> APSRANTKVIVVGGGGTIGSSTALHLVRSGYTPSNVTVLDAYPIPSCQSAGNDLNKIMDADADPAADAARQMWNEDELFKKFFHNTGRLDCAHGEKDIADLKKRYQNLVDWGLDATVEWLDSEDEILKRMPQLTRDQIKGWKAIFSKDGGWLAAAKAIKAIGEYLRDQGVRFGFYGAGSFKQPLLAEGVCIGVETVDGTRYYADKVVLAAGAWSPTLVELQEQCVSKAWVYGHIQLTPEEAARYKNSPVVYNGDVGFFFEPNEHGIIKVCDEFPGFTRFKMHQPFGAKAPKRISVPRSHCKHPTDTIPDASIVRIRRAIATFMPQFKNKPLFNQAMCWCTDTADGHLLICEHPEWKNFYLATGDSGDSFKLLPIIGKYVVELLEGTLADELAHKWRWRPGSGDALKSRREAPAKDLADMPGWNHD

Fructosyl peptide oxidases (FPOX) are deglycating enzymes that find application as key enzymatic components in diabetes monitoring devices. The inability of wild type FPOXs to act on intact proteins is the most critical issue limiting both their diabetes detection efficiency and their protein deglycation potential. This is due to their buried active site and narrow access tunnel, as determined in multiple crystal structures. In that account, using a rational design approach involving a five-amino acid deletion at the entrance of the active site and a number of further mutations, we described a stable PnFPOX mutant (named L3-35A) that, relative to the wild type enzyme, features a significantly wider and shorter access tunnel.

In the present study, we set out to enhance the thermal stability of the L3-35A mutant by implementing a methodological approach whereby different thermal stabilization strategies are tested in parallel and their efficiency compared. These various strategies involved mutations to either improve the RMSF of the protein (generating mutants hereafter referred to as D-series mutants), increase the number of salt bridges (C-series mutants) or form disulfide bonds (X-series mutants). Our MD-based ranking led to the selection of six candidate mutants (C16, D02, X01, X02A, X04, and X07) for experimental production and characterization. On the other hand, the introduction of extensive surface charges and salt bridges (mutant C16) resulted in a further increase in Tm of ≈ 1.5 °C (Tm = 55.2 °C). Finally, the incorporation of a single disulfide bond in different positions on the L3-35A scaffold led to a significant improvement in thermal stability of all the tested mutants of this series: X01 (54.1 °C), X02 (60.0 °C), X04 (55.2 °C) and X07 (55.3 °C). In particular, we have shown that the introduction of a disulfide bond allowed us to produce a PnFPOX variant that shows remarkably higher thermal stability compared to the other mutants. Based on our thermostability results, we selected the X02A variant for its high Tm, high expression yield, and detectable activity toward glycated amino acids and we set out to increase its activity toward larger substrates (i.e., fVH and F6P). The activity toward these substrates was present in the wild type enzyme PnFPOX but was lost in the L3-35A design. In this process, while the amino acids that are directly involved in the catalytic function were not modified, some tunnel-lining residues were replaced. This could explain the reduced activity of both the L3-35A enzyme previously reported and its thermally-stabilized mutants described so far (D02, C16, X01, X02A, X04, X07). Hence, we set out to design mutations to enhance the catalytic activity of X02A, the most thermally-stable mutant of our library.> MCYTGDPANNPLDRVRILCTDTDNNEILID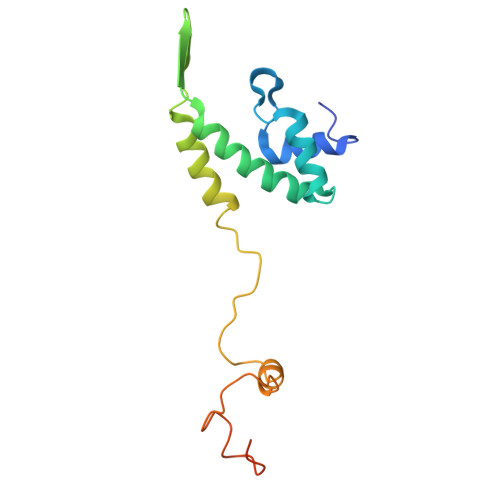QSVLEWFYQESGKDEKKAAIKALKYLLFQVAKMGDEKVGGVYLRNSSRFKSLKAVYDDLVKSSVSGLPYAGGINQCDIDMRRQNPCSVKKYTEYGDAVRYYGRDYCERVNGVFIIERDE> STAGKVIKCKAAVLWEEKKPFSIEEVEVAPPKAHEVRIKMVATGICRSDDHVVSGTLVTPLPVIAGHEAAGIVESIGEGVTTVRPGDKVIPLFTPQCGKCRVCKHPEGNFCLKNDLSMPRGTMQDGTSRFTCRGKPIHHFLGTSTFSQYTVVDEISVAKIDAASPLEKVCLIGCGFSTGYGSAVKVAKVTQG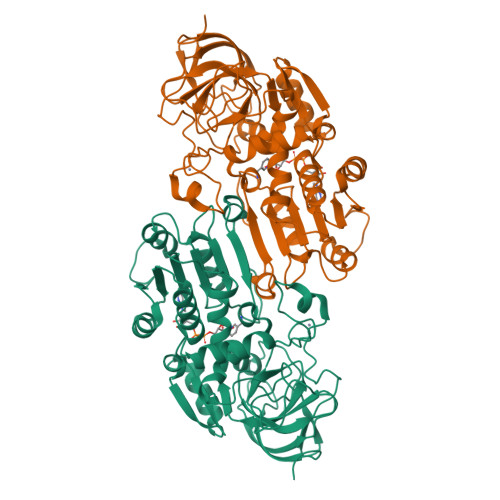STCAVFGLGGVGLSVIMGCKAAGAARIIGVDINKDKFAKAKEVGATECVNPQDYKKPIQEVLTEMSNGGVDFSFEVIGRLDTMVTALSCCQEAYGVSVIVAVTPDSQNLSMNPMLLLSGRTWKGAIFGGFKSKDSVPKLVADFMAKKFALDPLITHVLPFEKINEGFDLLRSGESIRTILTF>[6x]MAMSQQDLPTLFYSGKSNSAVPIISESELQTITAEPWLEISKKGLQLEGLNFDRQGQLFLLDVFEGNIFKINPETKEIKRPFVSHKANPAAIKIHKDG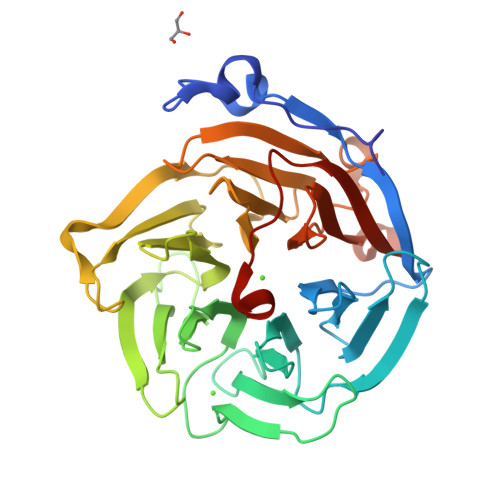RLFVCYLGDFKSTGGIFAATENGDNLQDIIEDLSTAYCINDMVFDSKGGFYFTDFRGYSTNPLGGVYYVSPDFRTVTPIIQNISVANGIALSTDEKVLWVTETTANRLHRIALEDDGVTIQPFGATIPYYFTGHEGPDSCCIDSDDNLYVAMYGQGRVLVFNKRGYPIGQILIPGRDEGHMLRSTHPQFIPGTNQLIICSNDIEMGGGSMLYTVNGFAKGHQSFQFQLEHHHHHH>EEVTIKANLIFANGSTQTAEFKGTFEKATSEAYAYADTLKKDNGEWTADVADKGYTLNIKFAG[4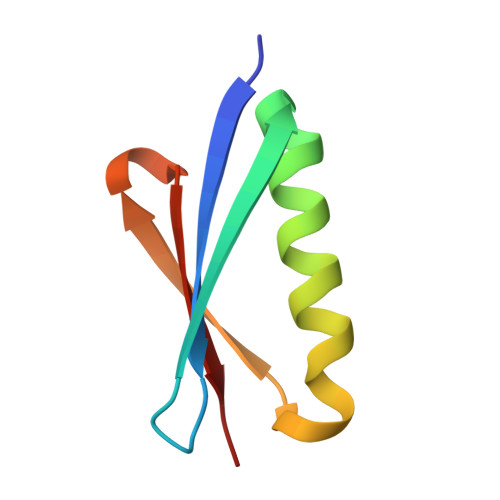x]> GSYNKPSETVIPESVDGLQE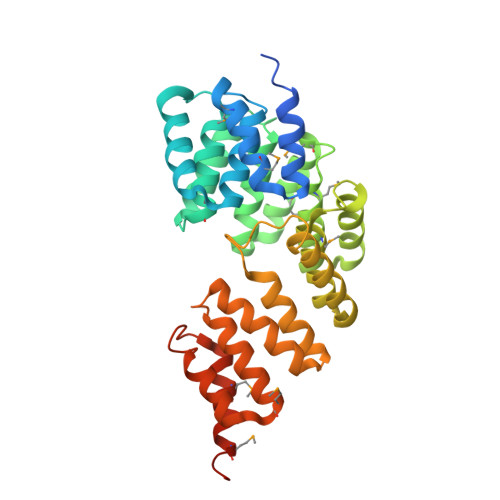NLDVVVSLAERHYYNCDFKMCYKLTSVVMEKDPFHASCLPVHIGTLVELNKANELFYLSHKLVDLYPSNPVSWFAVGCYYLMVGHKNEHARRYLSKATTLEKTYGPAWIAYGHSFAVESEHDQAMAAYFTAAQLMKGCHLPMLYIGLEYGLTNNSKLAERFFSQALSIAPEDPFVMHEVGVVAFQNGEWKTAEKWFLDALEKIKAIGNEVTVDKWEPLLNNLGHVCRKLKKYAEALDYHRQALVLIPQNASTYSAIGYIHSLMGNFENAVDYFHTALGLRRDDTFSVTMLGHCIEMYIGDSEAYIGADIK>[4x]MTNQKFFTLSNGNKIPAVAVVGTGTKWAHAEETDATFSQELTDIVKLSLDTVPGIVHIDAAEMYKTYPELGAALKETKKPREEIFITDKF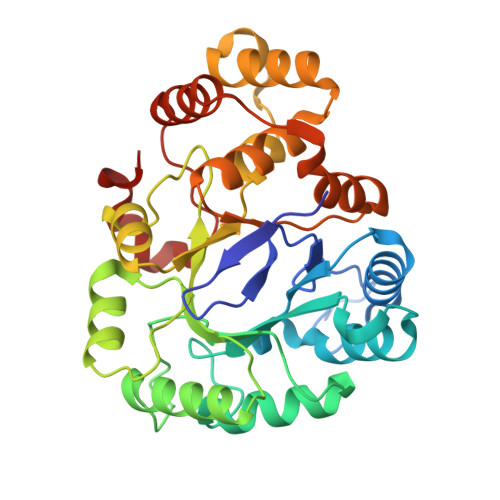SSLHKISEDPKSALETALNKLGVDYVDLYLIHSPFFDKDLNIDLETAWKQLEELYKSGKAKNIGVSNFTVEDLKKVLAIAEIKPQVNQIEFSPFLQNQTPGIVEFSQKNDILLEAYSPLGPLQKKPTDADQQPFYQYLKELSEKYNKTEAQVLLLWVYKRGILPVTTSAKIERIKQAQDIFSFDLTEEEVKKITDLGLQHEPVRLWHVDFYTKYNSEAQK>[2x]MYGITSTANSTGNQSYANRLFIYEVVGLGGDGRNENSLVRKSGTTFITVPYARMNQEMQRITKLGGKIVSIRPAEDAAQIVSEGQSSAQASAQSPMASSTKIVHPKTTDTSVPVNIYRPKTPFLGKCIENYELVDEGGSGTVRHVTFDISEGDLRYLEGQSIGIIPPGEDKNGKPHKLRLYSIASTRHGDMEDNKTVSLCVRQLEYQDPESGETVYGVCSTYLCNLPVGTDDVKITGPVGKE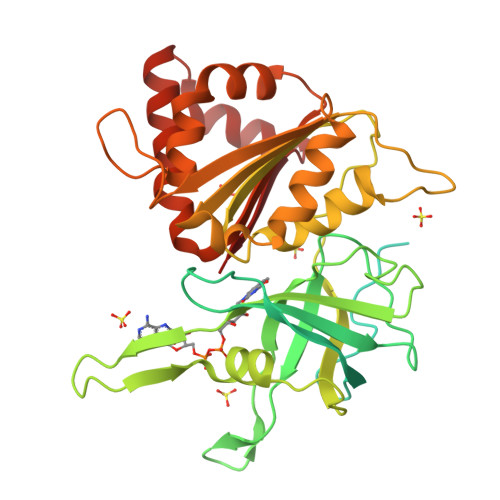MLLPDDEDATVVMLATGTGIAPFRAFLWRMFKEQHEDYKFKGKAWLIFGVPYTANILYKDDFEKMAAENPDNFRLTYAISREQKTADGGKVYVQSRVSEYADELFEMIQKPNTHVYMCGLKGMQPPIDETFTAEAEKRGLNWEEMRRSMKKEHRWHVEVY We here-report work carried out on PilO2Bp, a component of the Tfpb R64 thin pilus variant assembly machinery from B. pseudomallei. We show that N-PilO2Bp consists of two α/β sub-domains separated by a prominent central cleft, typical of actin-like ATPases. The function of PilO2 within the Tfpb assembly machinery is not documented, however, PilO2 is reported to be an assembly protein that localizes in the cytoplasm in the absence of other Pil proteins, translocating to the OM in their presence. FFPred, from the PSIPRED website, predicted the most plausible topology, with a cytoplasmic localization for the N-terminal domain (1-194), a transmembrane domain (195-214), and a periplasmic localization for the C-terminal domain (215-432).

Moreover, we report the 1.55 Å crystal structure of the N-terminal domain of PilO2Bp (residues 1-192; N-PilO2Bp), solved by S-SAD phasing, providing a first glimpse of the 3D structural properties of the PF06864 family, previously lacking a structure representative. Thus, considering the availability of 1.5 Å resolution data for this protein, the single-wavelength anomalous diffraction (SAD) phasing method was adopted based on the four intrinsic sulphur atoms present in native N-PliO2Bp. Four sulphur and one phosphor anomalous scatterers were located during the phasing procedure. The N-PilO2Bp 3D structure was then refined using data at 1.55 Å resolution, to R-free and R-factor values of 0.186 and 0.223, respectively (for further information see Materials and Methods). The first ‘dimeric’ interface, results from the interaction of two N-PilO2Bp molecules via a phosphate ion. Indeed, the identified phosphate ion is located in a pocket in the C-terminal region, interacting with Arg61, Arg189 and Asp42. In the crystal, the phosphate ion further interacts with Arg50 and Arg77 of a symmetry-related molecule. Considering the location of the expected transmembrane segment that follows N-PilO2Bp C-terminal residues, such positively charged surface may help the protein interact with a phosphate from IM phospholipid head groups. The second crystal packing dimer is built around an ‘anchor loop’ that covers residues 168-179. This loop was refined with higher than average B-factors, suggesting conformational flexibility that may mediate PilO2Bp interaction/recognition with other assembly machinery partners.

> YTMSAQVIQIGRQRFVGGLFWQSLSRRNELRAEAVELAKKLKFDLMVLRIDRGVAAAGYANTRDGFAPGHLSLGAMVSRAIALEGAFYNGRRQPAPNWLGAFALPDGRWAYFAVRDHAFMPNGDWVGSREEALERLHTDYAWGGWNVVIGEPELERQGFQNFQPKRLDDLLPRRGGRPRTERWWALRPVERRLS>AEFHHHHHHKDAPVLTKTFVDRINQLNGGMWKAVYNGKMQNITFAEAKRLTGAWIQKTSSLPPVRFTEEQLRTELPESFDSAEKWPNCPTIREIADQSACRASWAVSTASVISDR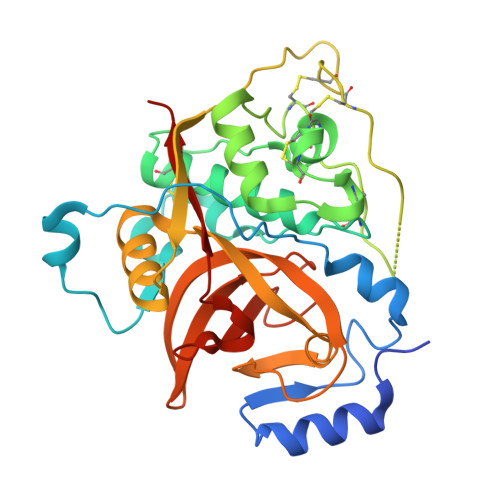YCTVGGVQQLRISAAHLLSCCKQCGGGCKGGFPGFAWRYYVEYGIASSYCQPYPFPHCEHRGAQGNKTPCSKYNFDTPKCQATCTDKSIPLVKYRGSATYLLLHGEEDYKRELYFNGPFVAVFYVYTDLFAYKSGVYRHVDGDFLGGTAVKVVGWGKLNGTPYWKVANTWDTDWGMDGYLLILRGNNECNIEHLGFAGTPETSQLT[3x]N-{5-[(3S)-3-(2-hydroxypropan-2-yl)pyrrolidin-1-yl]-2-(trifluoromethyl)pyridin-3-yl}-6-(1-methyl-1H-pyrazol-4-yl)pyridine-2-carboxamide 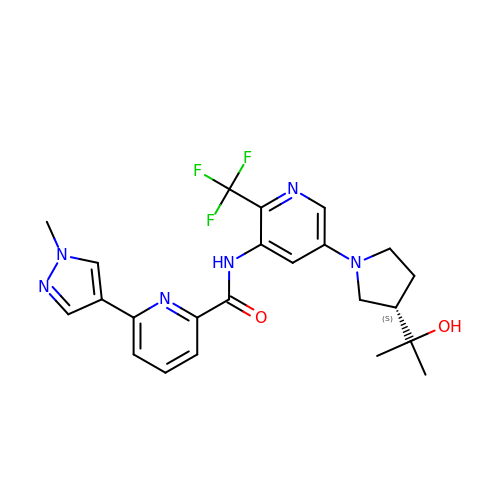| C23 H25 F3 N6 O2 | VNRCXZCFCYFZQN-HNNXBMFYSA-N> EAPHLVQVDA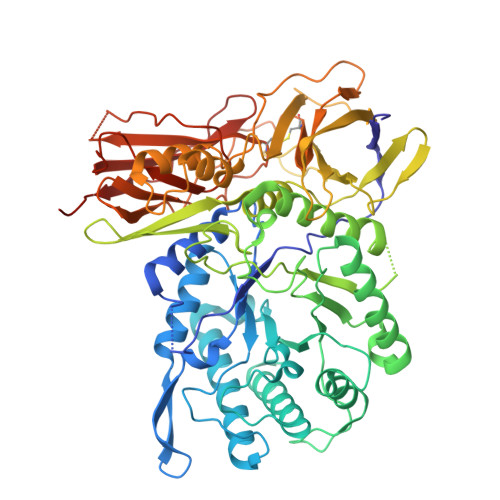ARALWPLRRFWRSTGFCPPLPHSQADPYVLSWDQQLNLAYVGAVPHRGIKQVRTHWLLELVTTRGSTGRGLSYNFTHLDGYLDLLRENQLLPGFELMGSASGHFTDFEDKQQVFEWKDLVSSLARRYIGRYGLAHVSKWNFETWNEPDHHDFDNVSMTMQGFLNYYDACSEGLRAASPALRLGGPGDSFHTPPRSPLSWGLLRHCHDGTNFFTGEAGVRLDYISLHRKGARSSISILEQEKVVAQQIRQLFPKFADTPIYNDEADPLVGWSLPQPWRADVTYAAMVVKVIAQHQNLLLANTTSAFPYALLSNDNAFLSYHPHPFAQRTLTARFQVNNTRPPHVQLLRKPVLTAMGLLALLDEEQLWAEVSQAGTVLDSNHTVGVLASAHRPQGPADAWRAAVLIYASDDTRAHPNRSVAVTLRLRGVPPGPGLVYVTRYLDNGLCSPDGEWRRLGRPVFPTAEQFRRMRAAEDPVAAAPRPLPAGGRLTLRPALRLPSLLLVHVCARPEKPPGQVTRLRALPLTQGQLVLVWSDEHVGSKCLWTYEIQFSQDGKAYTPVSRKPSTFNLFVFSPDTGAVSGSYRVRALDYWARPGPFSDPVPYLEVPVPRGPPSPGNP> MGSSHHHHHHSSGLVPRGSHSTQVAKKILVTCALPYANGSIHLGHMLEHIQADVWVRYQRMRGHEVNFICADDAHGTPIMLKAQQLGITPEQMIGEMSQEHQTDFAGFNISYDNYHSTHSEENRQLSELIYSRLKENGFIKNRTISQLYDPEKGMFLP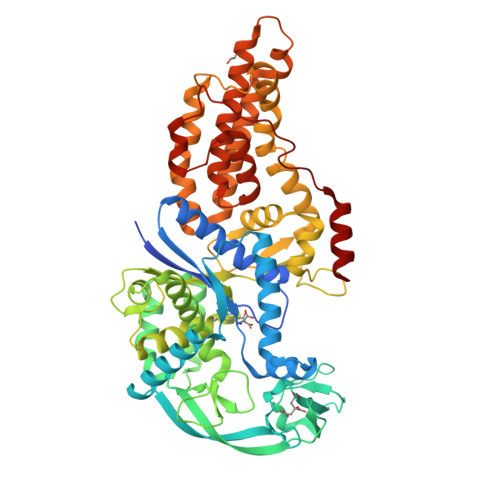DRFVKGTCPKCKSPDQYGDNCEVCGATYSPTELIEPKSVVSGATPVMRDSEHFFFDLPSFSEMLQAWTRSGALQEQVANKMQEWFESGLQQWDISRDAPYFGFEIPNAPGKYFYVWLDAPIGYMGSFKNLCDKRGDSVSFDEYWKKDSTAELYHFIGKDIVYFHSLFWPAMLEGSNFRKPSNLFVHGYVTVNGAKMSKSRGTFIKASTWLNHFDADSLRYYYTAKLSSRIDDIDLNLEDFVQRVNADIVNKVVNLASRNAGFINKRFDGVLASELADPQLYKTFTDAAEVIGEAWESREFGKAVREIMALADLANRYVDEQAPWVVAKQEGRDADLQAICSMGINLFRVLMTYLKPVLPKLTERAEAFLNTELTWDGIQQPLLGHKVNPFKALYNRIDMRQVEALVEASK> MSTCPIDPPALRAAFAGPLD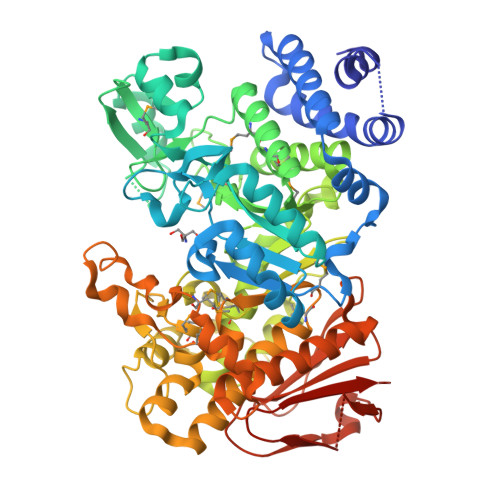PQHAEVLLSRYDQHASRLLDALHALYGQRADYASWLAQWLGEVGDIARQRPQALQTLDSTRHAGWFGQPHMLGYSAYADRFAGTLQGVAERVPYLQELGVRYLHLLPFLRARAGDNDGGFAVSDYGQVEPSLGSNDDLVALTSRLREAGISLCADFVLNHTADDHAWAQAARAGDARYLDYYHHFADRTVPDRYEATLGQVFPHTAPGNFTWVDDTAQWMWTTFYPYQWDLNWSNPAVFGDMALAMLRLANLGVEAFRLDSTAYLWKRIGTDCMNQSEAHTLLVALRAVTDIVAPAVVMKAEAIVPMTQLPPYFGSGVDEGHECHLAYHSTLMAAGWSALALQRGDILHNVIAHSPPLPRHCAWLSYVRCHDDIGWNVLQHEACGNAAQPPFSLRDVARFYANAVPGSYARGESFQSSGDGVHGTNGMAAALAGIQAAQEAGDAAALAVAVDRLVLLYAIALAMPGVPLIYMGDELAMVNDPGYRDDPHRQHEGRWLHRPAMDWQLAAQRHDAKSLSGTVYRRLRGLIRQRAALGALAADQALASIALNDPRVFALTRGDSFIALHNFSDQLLDVELAAIGVDGWTLLAIDDAIGGAAARGDGSIVLPPYGVRWLQRGTEHAPE>[4x]MHHHHHHMSNPQPEKVRVVVGDDHPLFREGVVRALSLSGSVNVVGEADDGAAALELIKAHLPDVALLDYRMPGMDGAQVAAAVRSYELPTRVLLISAHDEPAIVYQA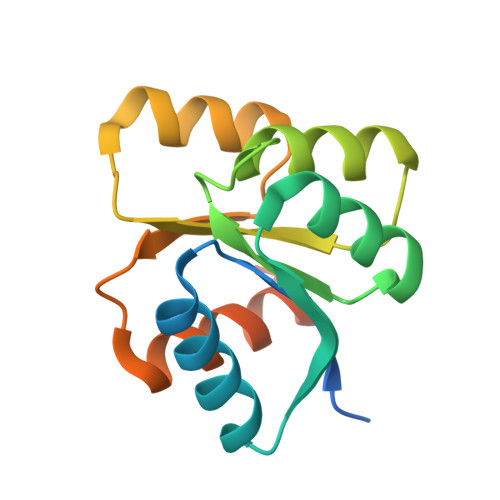LQQGAAGFLLKDSTRTEIVKAVLDCAKGRDVVAPSLVGGLAGEIR> XAFAGILADADCAAAVKACEAADSFSYKAFFAKCGLSGKSADDIKKAFVFIDQDKSGFIEEDEL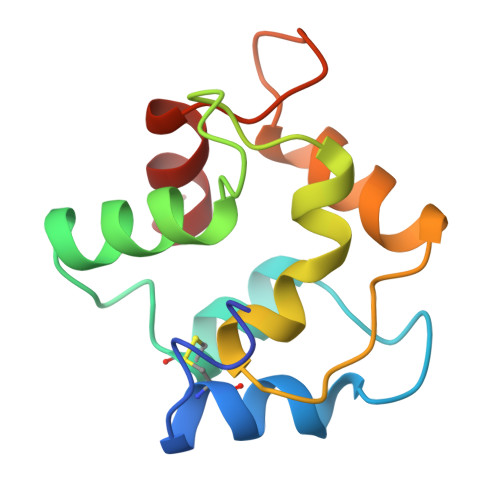KLFLQVFKAGARALTDAETKAFLKAGDSDGDGAIGVEEWVALVKA>GPLGSTEVLCLMNMVLPEELLDDEEYEEIVEDVR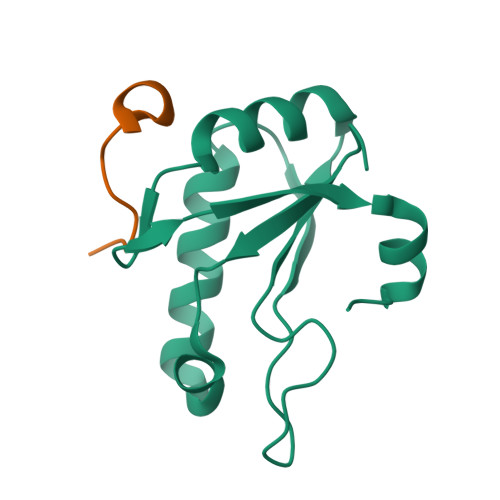DECSKYGLVKSIEIPRPVDGVEVPGCGKIFVEFTSVFDCQKAMQGLTGRKFANRVVVTKYCDPDSYHRRDFW[2x];>KRKSRWDETPASQMGGSTP[2x]k-Junctions are elaborated forms of kink turns with an additional helix on the nonbulged strand, thus forming a three-way helical junction. k-junctions are elaborated forms of k-turns, preserving the tandem G:A base pairs and cross-strand hydrogen bonding, but having an additional third helix on the n (nonbulged) strand opposite the loop on the b (bulged) strand. One quite widespread junction is the kink-turn (k-turn); a motif commonly found in duplex RNA comprising a short (usually 3 nt) bulge-loop followed by conserved G:A and A:G sheared base pairs (Klein et al. 2001). k-turns can be induced to fold (e.g., by addition of metal ions) into a tightly kinked structure with an included angle of ∼50°, stabilized by critical cross-strand hydrogen bonds between 2′-hydroxyl groups and ring nitrogen atoms of the adenine nucleobases of the G:A base pairs. In addition to these k-turns, we also identified a candidate k-junction in a sequence termed DUF-3268.

We synthesized a single 46 nt RNA oligonucleotide containing a DUF-3268 k-junction, with both the NC- and T-helices terminated by GAAA tetraloops. This crystallized in space group C121, and diffracted to a resolution of 1.94 Å. The overall architecture of the DUF-3268 k-junction is very similar to that of the Arabidopsis and E. coli k-junctions, forming a three-way helical junction in which the C- and T-helices are coaxial, and the axis of the NC-helix includes an acute angle with that of the C-helix. As predicted, the O2′ of the ribose designated L1 donates a hydrogen bond to A1n N1. Similarly, the O2′ of the ribose assigned as −1n donates a hydrogen bond to A2b N1. The RNA conformation corresponds to that of an N1-type k-turn, that is, A2b accepts a proton at N1. The first connecting nucleotide c1 forms a cis Watson–Crick C:G base pair with L1. Instead of base pairing with L1.1 it is extended out, and UL1.1 forms an in-plane triple base interaction with the major groove edge of the junction-proximal base pair of the T-helix. In the DUF-3268 k-junction there is no nucleotide inserted between G1b and A2b.

> GGGAGUUAGACUCGCGAAAGCGAGGAACUGCGAAAGCAGUACUUCC> GKIGIFFGTDSGNAEAIAEKISKAIGNAEVVDVAKASKEQFNGFTKVILV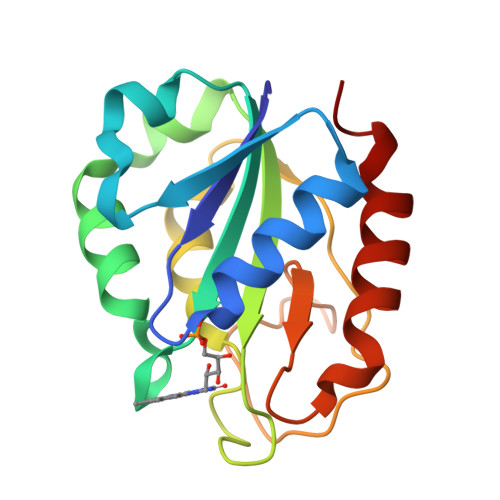APTAGAGDLQTDWEDFLGTLEASDFANKTIGLVGLGDQDTYSETFAEGIFHIYEKAKAGKVVGQTSTDGYHFAASKAVEGGKFVGLVIDEDNQDDLTDERIAKWVEQVRGSFA>[2x]GPSFWLGNETLKVPLALFALNRQRLCERLRKNPAVQAGSIVVLQGGEETQRYCTDTGVLFRQESFFHWAFGVTEPGCYGVIDVDTGKSTLFVPRLPASHATWMGKIHSKEHFKEKYAVDDVQYVDEIASVLTSQKPSVLL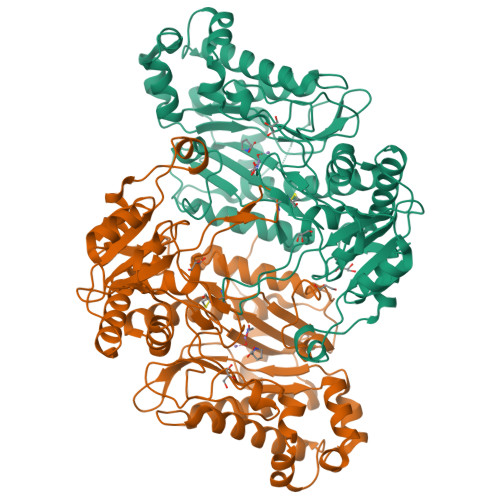TLRGVNTDSGSVCREASFDGISKFEVNNTILHPEIVECQVFKTDMELEVLRYTNKISSEAHREVMKAVKVGMKEYELESLFEHYCYSRGGMRHSSYTCICGSGENSAVLHYGHAGAPNDRTIQNGDMCLFDMGGEYYCFASDITCSFPANGKFTADQKAVYEAVLRSSRAVMGAMKPGVWWPDMHRLADRIHLEELAHMGILSGSVDAMVQAHLGAVFMPHGLGHFLGIDVHDVGGYPEGVERIDEPGLRSLRTARHLQPGMVLTVEPGIYFIDHLLDEALADPARASFLNREVLQRFRGFGGVRIEEDVVVTDSGIELLTCVPRTVEEIEACMAGCDKAFTPFS>[8x]MGSSHHHHHHSSGLVPRGSMNIFDVKDKYILITGASSGLGHHIAELFAKEGANIVICARRLERLKELESHIKNEYGVQVYTFALDVNDRSAVKDMLSSLEAEGVTIDVLINNAGVSDTKRFLDYNDEDWDKIVDTNLKAPWQCAQEVVQHMIKAERKGSIINITSILSQSTNLGVSPYCASKAGLRHLTEVMAVELARFGINVNAIAPGYMITEINEEYLTSEVGQQLLKKIPTRKFVEFDD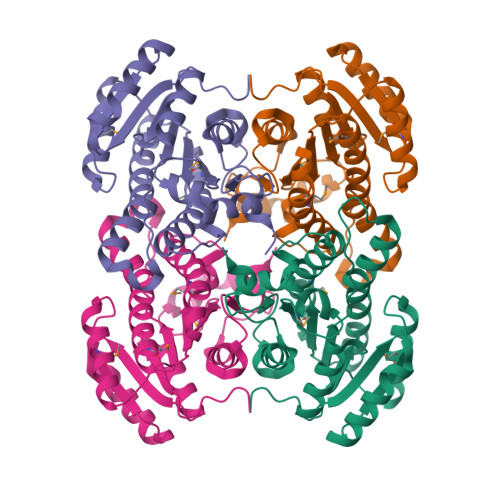LNGPLLLLASQAGQGITGIEIKVDGGHSAAPI>[4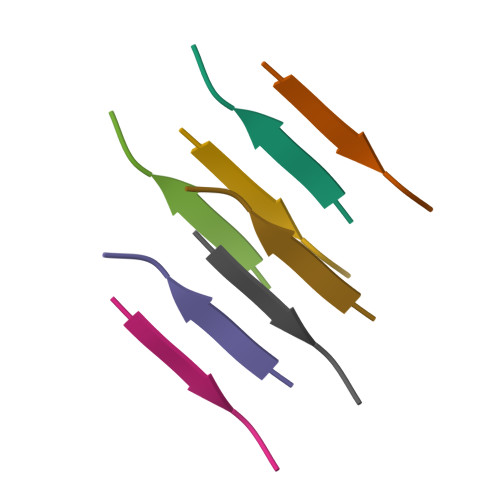x]LSFSKD>[2x]HHHHHHSSGLVPRGSMTATETVRVRFCPSPTGTPHVGLVRTALFNWAYARHTGGTFVFRIEDTDAQRDSEESYLALLDALRWLGLDWDEGPEVGGPYGPYRQSQRAEIYRDVLARLLAAGEAYHAFSTPEEVEARHVAAGRNPKLGYDNFDRHLTDAQRAAYLAEGRQPVVRLRMPDDDLAWNDLVRGPVTFAAGSVPDFALTRASGDPLYTLVNPCDDALMKITHVLRGEDLLPSTPR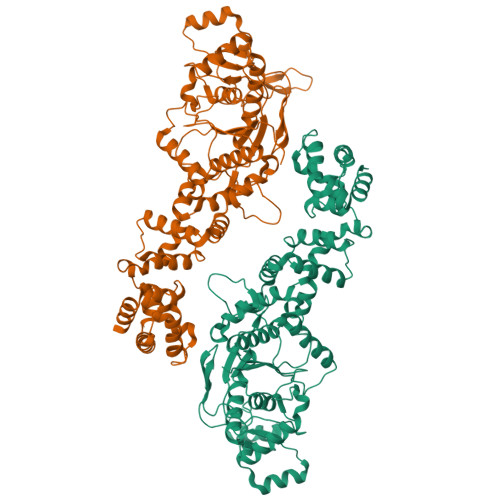QLALHQALIRIGVAERIPKFAHLPTVLGEGTKKLSKRDPQSNLFAHRDRGFIPEGLLNYLALLGWSIADDHDLFGLDEMVAAFDVADVNSSPARFDQKKADALNAEHIRMLDVGDFTVRLRDHLDTHGHHIALDEAAFAAAAELVQTRIVVLGDAWELLKFFNDDQYVIDPKAAAKELGPDGAAVLDAALAALTSVTDWTAPLIEAALKDALIEGLALKPRKAFSPIRVAATGTTVSPPLFESLELLGRDRSMQRLRAARQLVGHA> NSDSECP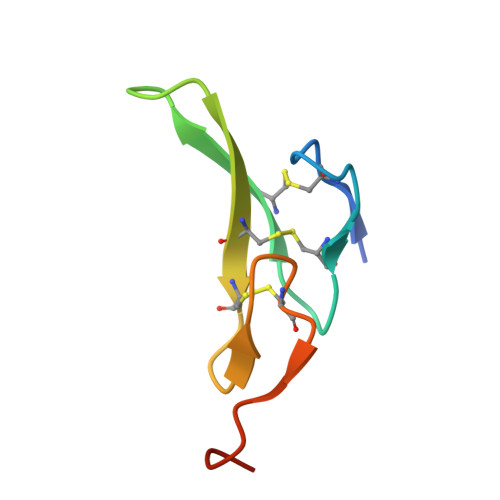LSHDGYCLHDGVCMYIEALDKYACNCVVGYIGERCQYRDLKWWELR> GSSSWNDIKNSGYISRYLTDFEPIQCLGRGGFGVVFEAKNKVDDCNYAIKRIRLPNRELAREKVMREVKALAKLEHPGIVRYFNAWLEAPPEKWQEKLQPSSPKVYLYIQMQLCRKENLKDWMNGRCTIEERERSVCL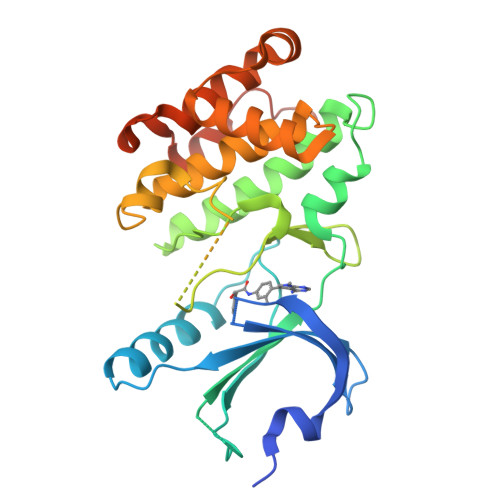HIFLQIAEAVEFLHSKGLMHRNLKPSNIFFTMDDVVKVGDFGLVTAMDQDEEEQTVLTPMPAYARHTGQVGTKLYMSPEQIHGNSYSHKVDIFSLGLILFELLYPFSTQMERVRTLTDVRNLKFPPLFTQKYPCEYVMVQDMLSPSPMERPEAINIIENAVFEDLDFPGKTVLRQRSRS> MTQCYAEITGWGKCLPPATLSNHDLSTFLDTSDEWIQSRTGIEQRRISHVNTSDLATVAAQHAIACAGVSVEEIDLIIVATCSPDSLIPNIASRVQQNLGIPSAAAFDLNAAATGFLYGLETATRLMQASHYRHALVIGAERLSFYLDWTKRDTAVLFGDGAGAVVLSKTEQKVGLQDAQIGCDAQGRDILAVPKFGTAMDRFDADNG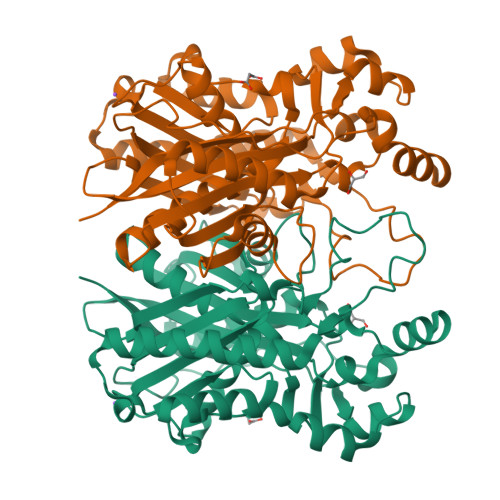YWAFDFVGKEIFKRAVRGMGAAAQQVLARSGLSTEEIDVVIPHQANIRIIQTLCDLAGIAQDKAFVNIHRYGNTSAATVPIALCEALEQGKIKPHDDLLVAAFGAGLTWGAGHIRWGERITPLGKSDAQLPSCDHTALDLLSKAIEHCKRHQSE> VPYKGYLIDLDGTIYQGKNRIPAGERFIKRLQERGIPYLLVTNNTTRTPEMV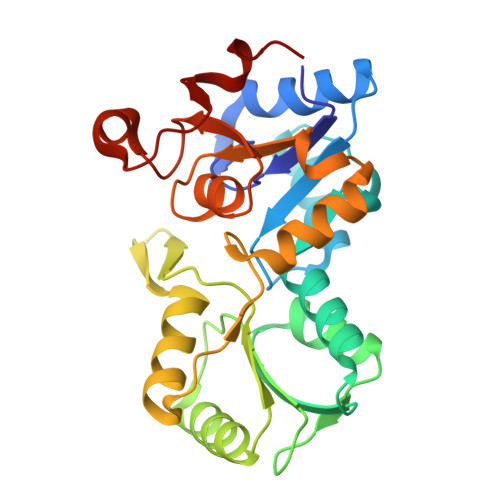QSMLANQFHVETSIETIYTATMATVDYMNDMNRGKTAYVIGETGLKSAIAAAGYVEELENPAYVVVGLDSQVTYEMLAIATLAIQKGALFIGTNPDLNIPTERGLMPGAGALNALLEAATRVKPVFIGKPNAIIMNKSLEVLGIQRSEAVMVGDNYLTDIMAGIQNDIATILVTTGFTRPEEVPTLPIQPDHVLSSLDEWRL> EFMVSLPRMVYPQPKVLTPCRKDVLVVT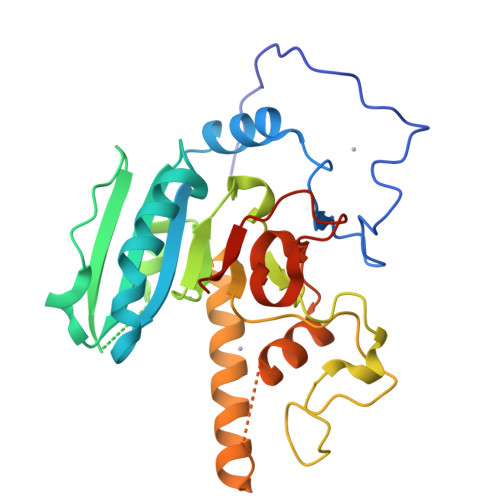PWLAPIVWEGTFNIDILNEQFRLQNTTIGLTVFAIKKYVAFLKLFLETAEKHFMVGHRVHYYVFTDQPAAVPRVTLGTGRQLSVLEVRAYKRWQDVSMRRMEMISDFCERRFLSEVDYLVCVDVDMEFRDHVGVEILTPLFGTLHPGFYGSSREAFTYERRPQSQAYIPKDEGDFYYLGGFFGGSVQEVQRLTRACHQAMMVDQANGIEAVWHDDSHLNKYLLRHKPTKVLSPEYLWDQQLLGWPAVLRKLRFTAVPKNHQAVRNPE> SHAPTRSARDIHQLEARIDSLAARNSKLMETLKEARQQLLALREEV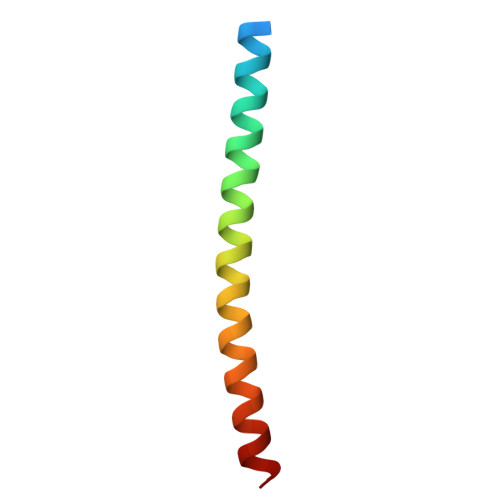DRLGQ>SNAASSFASVQAVVNKEYGLPEDYKPEDLVVPNVPFSFSGTLEKSYLRKEAAEALERLFDLANKEGIQLNAVSGFRSYDYQKKLYANNVKRKGQEHTDRFSAKPGHSEHQTGLTMDVSSKSANNELELTFANTKE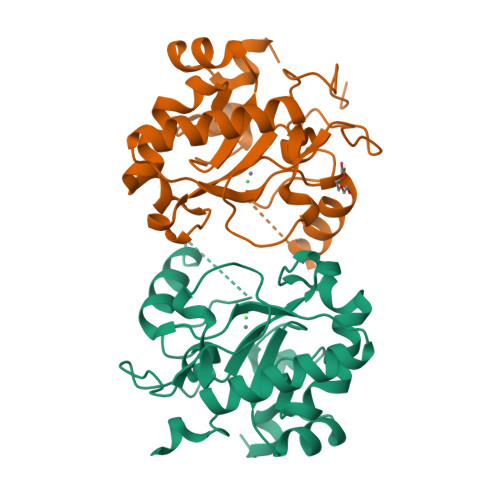GKWLKENAHRAGFIIRYPKGKESITGYAYEPWHIRYVGDIAESIYKKKLTLEEYMNL[2x]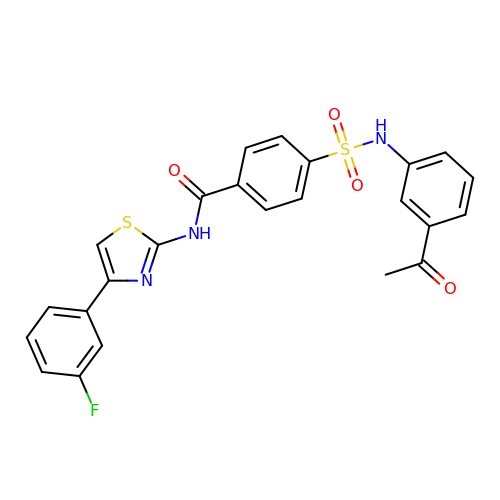4-[(3-ethanoylphenyl)sulfamoyl]-~{N}-[4-(3-fluorophenyl)-1,3-thiazol-2-yl]benzamide | C24 H18 F N3 O4 S2 | VUAMLKVINZWIJR-UHFFFAOYSA-N>MIWKRHLTLDELNATSDNTMVAHLGIVYTRLGDDVLEAEMPVDTRTHQPFGLLHGGASAALAETLGSMAGFMMTRDGQCVVGTELNATHHRPVSEGKVRGVCQPLHLGRQNQSWEIVVFDEQGRRCCTCRLGTA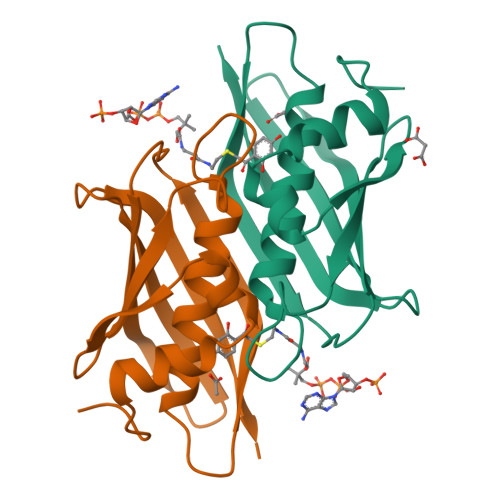VLG[2x]> AAMAFTLADRVTEEMLADKAALVVEVVEENYHDAPIVGIAVVNEHGRFFLRPETALADPQFVAWLGDETKKKSMFDSKRAAVALKWKGIELCGVSFDLLLAAYLLDPAQGVDDVRAAAKMKQYEAVRPDEAVYGKGAKRAVPDEPVLAEHLVRKAAAIWELERPFLDELRRNEQDRLLVELEQPLSSILAEMEFAGVKVDTKRLEQMGKELAEQLGTVEQRIYELAGQEFNINSPKQLGVILFEKLQLPVLKKTKTGYSTSADVLE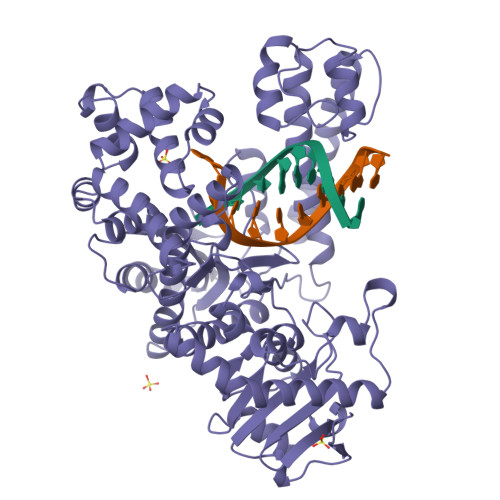KLAPYHEIVENILHYRQLGKLQSTYIEGLLKVVRPDTKKVHTIFNQALTQTGRLSSTEPNLQNIPIRLEEGRKIRQAFVPSESDWLIFAADYSQIELRVLAHIAEDDNLMEAFRRDLDIHTKTAMDIFQVSEDEVTPNMRRQAKAVNFGIVYGISDYGLAQNLNISRKEAAEFIERYFESFPGVKRYMENIVQEAKQKGYVTTLLHRRRYLPDITSRNFNVRSFAERMAMNTPIQGSAADIIKKAMIDLNARLKEERLQAHLLLQVHDELILEAPKEEMERLCRLVPEVMEQAVTLRVPLKVDYHYGSTWYDAK methyl 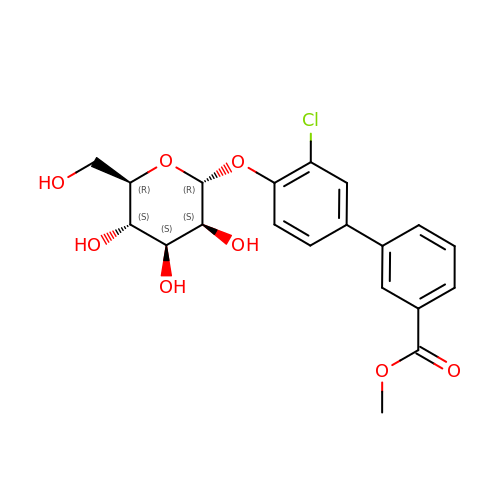3-[3-chloranyl-4-[(2~{R},3~{S},4~{S},5~{S},6~{R})-6-(hydroxymethyl)-3,4,5-tris(oxidanyl)oxan-2-yl]oxy-phenyl]benzoate | C20 H21 Cl O8 | PDLRSZVVAYSCAH-JGLNRKDHSA-N>NNTLWTGPKPEANCIIEYGKQNPDSKLTLILVKNGGIVNGYVTLMGASDYVNTLFKNKNVSINVELYFDATGHILPDSSSLKTDLELKYKQTADFSARGFMPSTTAYPFVLPNGTHNENYIFGQCYYKASDGALFPLEVTVMLNKRLPDSRTSYVMTFLWSLNAGLAPETTQATLITSPFTFSYIRED[3x];> PVFTQDVFVGSVEELSAAHTLVMKINATDAEPNTLSKISYRIVSLEPAYPPVFYLNKDTGEIYTTSVTLDREEHSSYTLTVEARDGVKQAQVQIRILDVNDNIPVVELEGMVEENQVNVEVTRIKVFDADEIGSDNWLANFTFASGNEGGYFHIETDAQTNEGIVTLIKEVYMKNLDFSVIVANKAAFHKSIRSKYKPTPIPIKVKVK

The first step of adenoviral replication involves the interaction of the fibre protein and more precisely the globular trimeric knob with an attachment receptor from the host cell. Desmoglein 2 (DSG2), a newly identified adenovirus receptor has been reported to be used by some species B human adenoviruses including HAd3, HAd7, HAd11 and HAd14 for cell infection. The intermediate portion of the DSG2 ectodomain, consisting of EC2 and EC3, has been described as important for recognition by the HAd3 knob (HAd3K), the trimeric globular distal part of the fibre protein. Here, we report the structure of HAd3 fibre knob (HAd3K) in complex with one and two molecules of the DSG2 receptor.

We recently demonstrated that HAd3K binds to DSG2 by a non-classical mechanism involving mainly one receptor bound per trimeric fibre knob. The interaction with DSG2 ectodomains (EC2 and EC3) takes place at the top of the trimeric HAd3K close to the three-fold axis. The EC2-EC3 domains span two HAd3K monomers, with the third monomer having no contacts with the receptor in the 1:1 complex. Each EC domain interacts with one monomer and targets primarily loop regions of HAd3K. In monomer ‘A’, the EC2 domain interacts with a surface exposed loop between the A and B strands and the C–D loop and N-terminal portion of the D strand. EC3 interacts with a loop between the G–H strands of monomer ‘B’. Several residues distributed along the EC2 primary sequence were found to interact with the HAd3K monomer, while only one region in EC3 (covering residues 311 to 321) is involved in the interaction with the groove of a second monomer. In the 1:1 HAd3K-DSG structure only a single monomer of HAd3K binds either the EC2 or EC3 domains. N186, V189 and S190 are at the interface between HAd3K and the EC2 module while L296, D261 or F265 are part of the HAd3K/EC3 module interface. Modeling of HAd3K binding to one DSG2 molecule in such an organized structure precludes the binding of a second DSG2 molecule coming either in cis or in trans without significant rearrangement of the desmosomal cadherins.>[2x]MPRL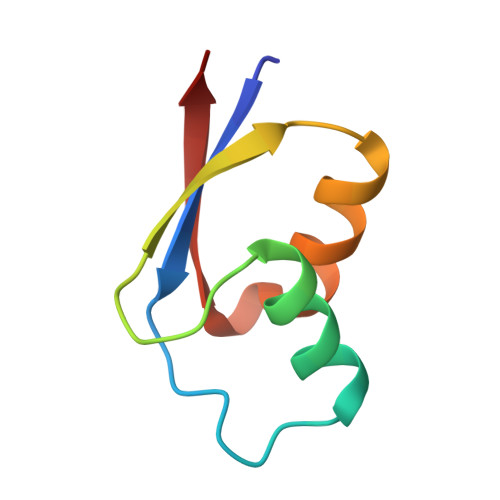KVKLVKSPIGYPKDQKAALKALGLRRLQQERVLEDTPAIRGNVEKVAHLVRVEVVE ethyl pyrazolo[1,5-a]pyridine-3-carboxylate | C10 H10 N2 O2 | 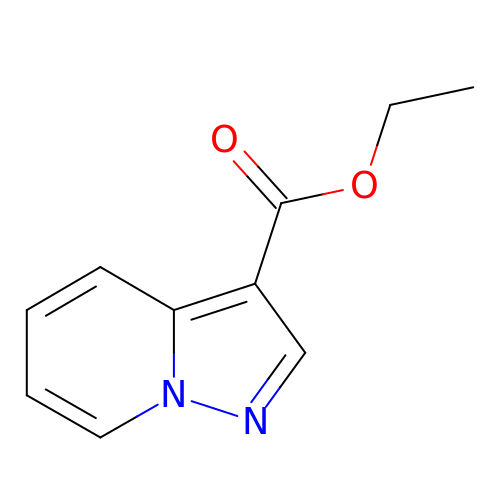IDHMFSBXNNIWCT-UHFFFAOYSA-N6-(4-CHLORO-2-HYDROXY-PHENOXY)-NAPHTHALEN-2-OL | C16 H11 Cl O3 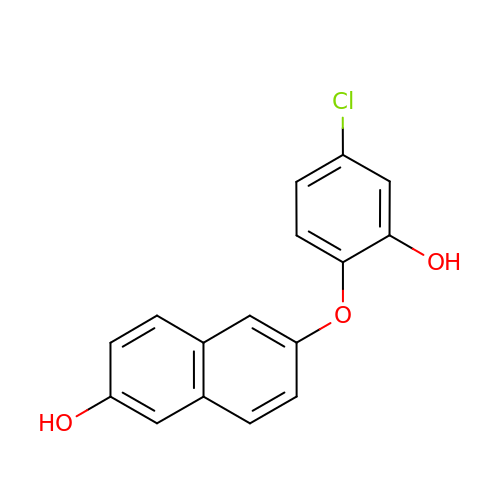| JPSDMABQCFCGLC-UHFFFAOYSA-N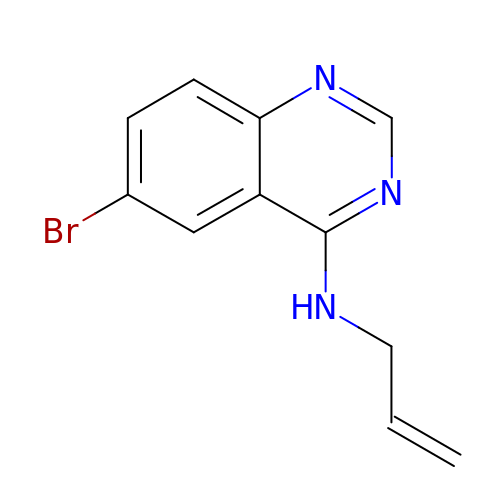6-bromo-N-(prop-2-en-1-yl)quinazolin-4-amine | C11 H10 Br N3 | BCPOLXUSCUFDGE-UHFFFAOYSA-N> XWKTIKGKTW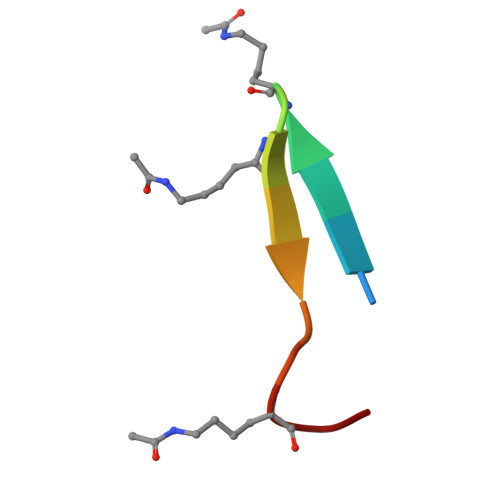RTKQC>[2x]MDQQGMVKKRLAVLVGCNYPNTRNELHGCINDVLAMKETILSRFGFKQDDIEVLTDEPESKVKPTGANIKAALRRMVDKAQAGSGDILFFHYSGHGTR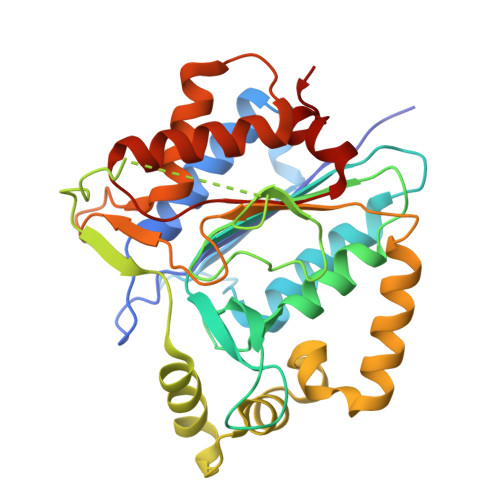IPSVKSAHPFKQDEAIVPCDFNLITDVDFRELVNQLPKGTSFTMISDSGHSGGLIDKEKEQIGPSSVSSNISPAIETTNKTITSRALPFKAVLDHLSSLTGITTSDIGTHLLELFGRDAGLKFRLPAMDLMDLLETMTAREKHVDSGILMSGCQADETSADVGVGNGKAYGAFSNAIQRVLNENEGAMKNKQLVMMARDVLERLGFHQHPCLYCSDQNADATFLSQP>MTKQEKTALNMARFIRSQTLTLLEKLNELDADEQADICESLHDHADELYRSCLASFKKNGQIDEQADICESLHDHADELYRSCLARFGGSKQEKTALNMARFIRSQTLTLLE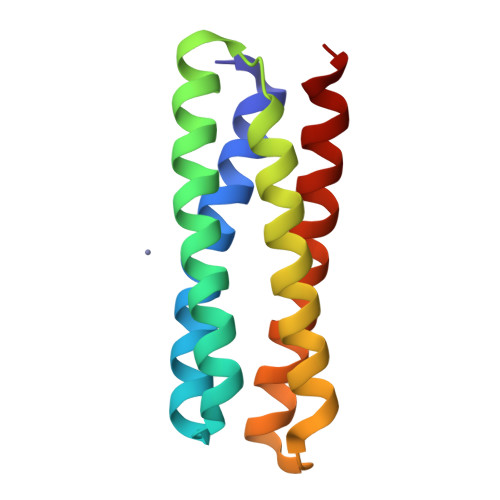KLNELAKG[2x]3-hydroxy-9,10-dioxo-9,10-dihydroanthracene-2-sulfonic acid | C14 H8 O6 S | 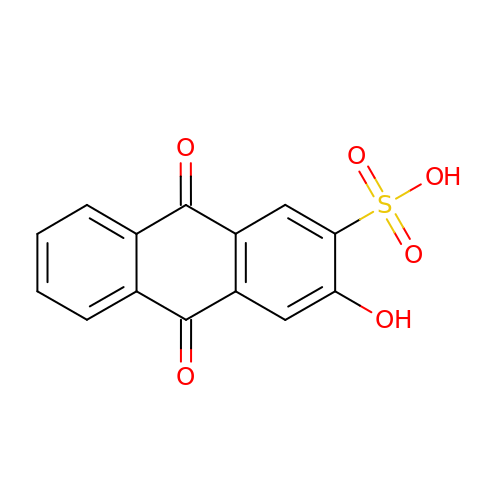PHPXXDWAMNINMC-UHFFFAOYSA-N> MSQDPKIVNPQLWPNPNKLRFADLYKYQGVEMKKINDSIKNYKAAKFYIGGILGGCLVFKFFIDAAVDKYIFGENGNGGKFLEMQTINSNYDYYYNRQFQRMRYLTEDPAGDDPLQKTKDEHLVDLGFIP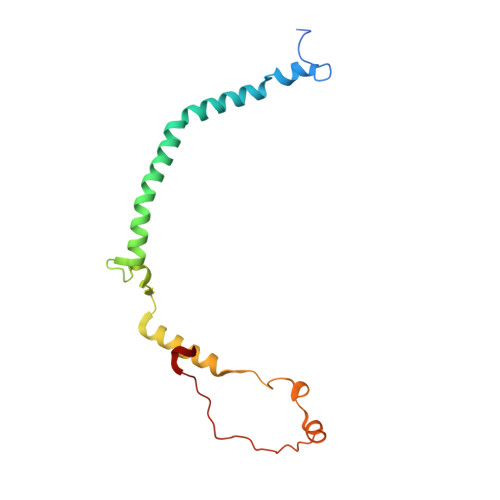KVFGANVEVRKRAPHDKYL> GQKKENYYVKHVEFPQSATIEQKVDMAARLVPTPQQYAWQQMELTAFLHFGINTFTGREWGDGKEDPALFNPSELDAEQWVRTLKEAGFKMVLLTAKHHDGFCLWPTATTKHSVASSPWKNGQGDVVKELRAACDKYDMKFGVYLSPWDRNAECYGDSPRYNDFFIRQLTELLTNYGEVHEVWFDGANGEGPN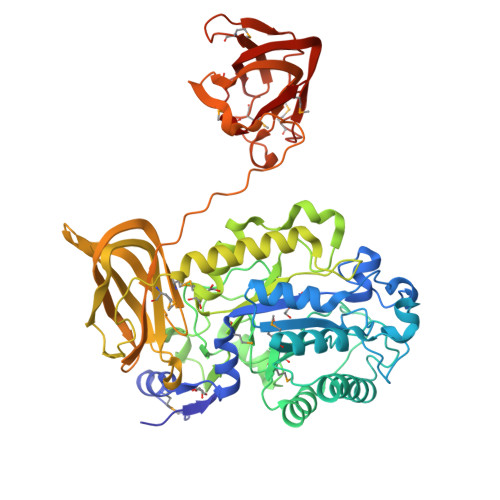GKKQVYDWDAFYQTIQRLQPKAVMAIMGDDVRWVGNEKGVGRETEWNATVLTPGIYARSQENNKRLGVFSKAEDLGSRKILEKATELFWYPSEVDVSIRPGWFYHAEEDGKVKSLKHLSDIYFQSVGYNSVLLLNIPPDRRGLIHEADIKRLKEFADYRQQTFADNRVKNGRKYWSTTSGGEAVYALKSKSEINLVMLQEDITKGQRVEAFTVEALTDNGWKEVGKGTTIGYKRMLRFPAVNANKLRVRIDECRLTAYVSQVAAYYAEPLQEETTKEDWNNLPRSGWKQVAASPLTIDLGKTVTLSSFTYAPSKAEVKPTMAFRYQFFVSMDGKSWKEVPASGEFSNIMHNPLPQTVAFSQKVQARFIKLEATTPDATVAKVNMNEIGVMVIP> MTENILRKSDEEIQKEITARVKALESMLIEQGILTTSMIDRMAEIYENEVGPHLGAKVVVKAWTDPEFKKRLLADGTEACMTENILRKSDEEIQKEITARVKALESMLIEQGILTTSMIDRMAEIYENEVGPHLGAKVVVKAWTDPEFKKRLLADGTEACKELGIGGLQGEDMMWVENTDEVHHVVVCTLCSCYPWPVLGLPPNWFKEPQYRSRVVREPRQLLKEEFGFEVPPSKEIKVWDSSSEMRFVVLPQRPAGTDGWSEEELAT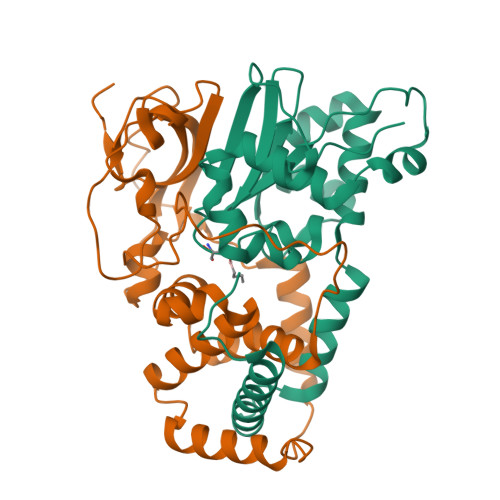LVTRESMIGVEPAKAVHHHHHH;> MNGVYDVGGTDGLGPINRPADEPVFRAEWEKVAFAMFPATFRAGFMGLDEFRFGIEQMNPAEYLESPYYWHWIRTYIHHGVRTGKIDLEELERRTQYYRENPDAPLPEHEQKPELIEFVNQAVYGGLPASREVDRPPKFKEGDVVRFSTASPKGHARRARYVRGKTGTVVKHHGAYIYPDTAGNGLGECPEHLYTVRFTAQELWGPEGDPNSSVYYDCWEPYIELVDTKAAAA>MKIAILSRDGTLYSCKRLREAAIQRGHLVEILDPLSCYMNINPAASSIHYKGRKLPHFDAVIPRIGTAITFYGTAALRQFEMLGSYPLNESVAIARARDKLRSMQLLARQGIDLPVTGIAHSPDDTSDLIDMVGGAPLVVKLVEGTQGIGVVLAETRQAAESVIDAFRGLNAHILVQEYIKEAQGCDIRCLVVGDEVVAAIERRAKEGDFRS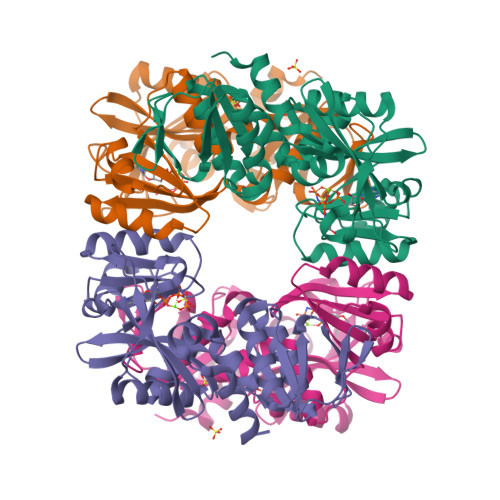NLHRGGAASVASITPQEREIAIKAARTMALDVAGVDILRANRGPLVMEVNASPGLEGIEKTTGIDIAGKMIRWIERHATTEYCLKTGGGTLVPR[8x]>[6x]SNAMDKYPFLREAGSSFKDRDVTKMSDLIATWDGQDIKGPALIGVPLSKSSISHSGASFAPGTIRQALKHSSAYSAELGEHVVSE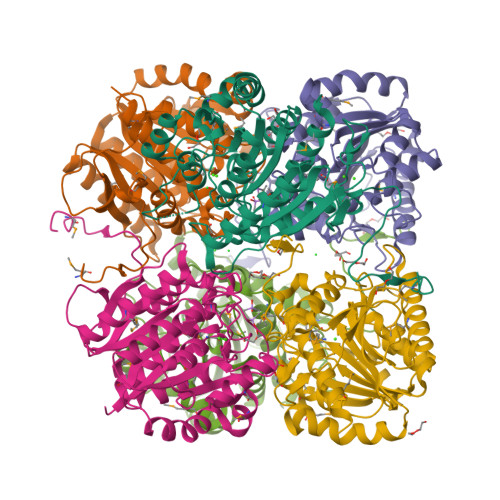LLYDLGDIDIHVTDIVKSHHHIFQTMHALLSDHPDWVPLILGGDNSISYSTIKAIAQTKGTTAVIQFDAHHDVRNTEDGGPTNGTPFRRLLDEEIIEGQHLIQLGIREFSNSQAYEAYAKKHNVNIHTMDMIREKGLIPTIKEILPVVQDKTDFIFISVDMDVLDQSHAPGCPAIGPGGLYTDELLEAVKYIAQQPNVAGIEIVEVDPTLDFRDMTSRAAAHVLLHALKGMKLSPFK> GSMVTAKNEDVLVNVEGGVGLLTLNRPKAINSLTHGMVTTMAERLAAWENDDSVRAVLLTGAGERGLCAGGDVVAIYHSAKADGAEARRFWFDEYRLNAHIGRYPKPYVSIMDGIVMGGGVGVGAHGNVRVVTDTTKMAMPEVGIGFIPDVGGTYLLSRAPGKLGLHAALTGAPFSGADAIVMGFAD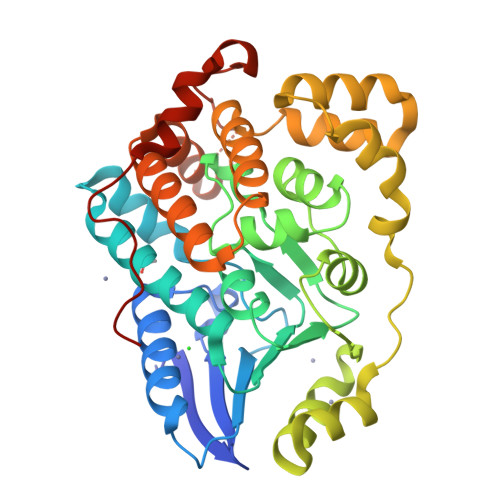HYVPHDKIDEFTRAVIADGVDAALAAHAQEPPASPLAEQRSWIDECYTGDTVADIIAALRAHDAPAAGEAADLIATRSPIALSVTLESVRRAAKLQSLEDTLRQEYRVSCASLKSHDLVEGIRAQLVDKDRNPKWRPATLAEVTEADVEAYFAPVDPELTFEGETQ> MEDEIRKAAEILAKSKH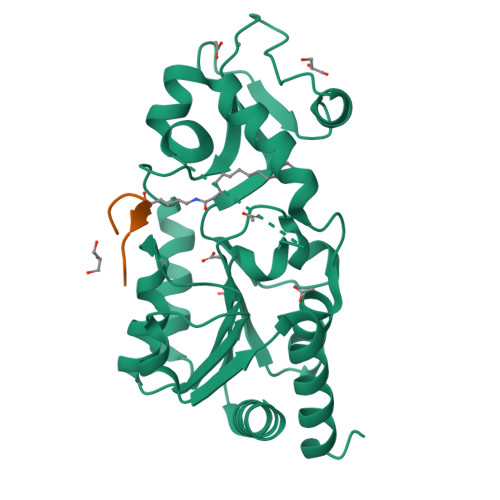AVVFTGAGISAESGIPTFRGEDGLWRKYDPEEVASISGFKRNPRAFWEFSMEMKDKLFAEPNPAHYAIAELERMGIVKAVITQNIDMLHQRAGSRRVLELHGSMDKLDCLDCHETYDWSEFVEDFNKGEIPRCRKCGSYYVKPRVVLFGEPLPQRTLFEAIEEAKHCDAFMVVGSSLVVYPAAELPYIAKKAGAKMIIVNAEPTMADPIFDVKIIGKAGEVLPKIVEEVKRLRSEK;> KGLGKGGAXRHRKW>[2x]GMAEQMRRVARLFGDWPETIIWTCLEGTMGDI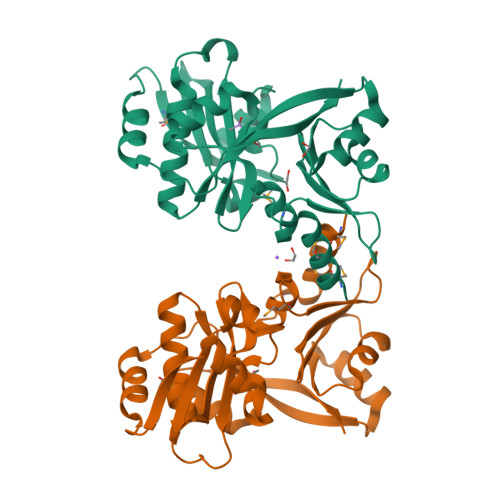YVDDSQSPQSALALYGRQSFFGFLAGQPHRDLLKICEGKNIILVPQNQAWSDLIEEVYGDGVRFFTRYATKKDTEFDLGHLQKLVDDLPESFDMKLIDRNLYETCLVEEWSRDLVGNYIDVEQFLDLGLGCVILHKGQVVSGASSYASYSAGIEIEVDTREDYRGLGLAKACAAQLILACLDRGLYPSWDAHTLTSLKLAEKLGYELDKAYQAYEWR>[4x]MRITLVDHPLVQHKLAHLRDKRTGPKDFRELAEEVAMLMAYEAMRDLELEETTVETPIAPARVKVLSGKK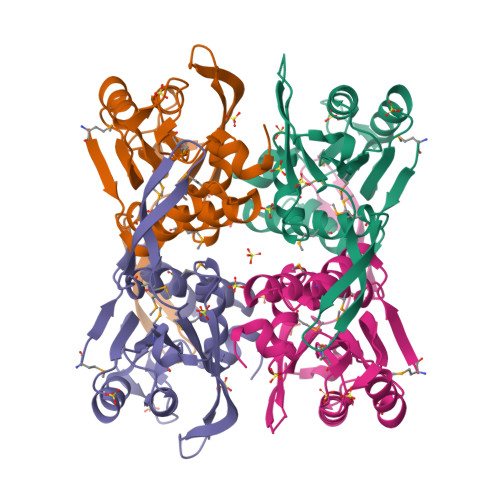LALVAILRAGLVMVEGILKLVPHARVGHIGLYRDPESLNPVQYYIKLPPDIAERRAFLLDPMLATGGSASLALSLLKERGATGVKLMAILAAPEGLERIAKDHPDTEVVVAAIDERLNDHGYIVPGLGDAGDRIYGTK> LPTSNPAQELEARQLGRTTRDDLINGNSASCADVIFIYARGSTETGNLGTLGPSIASNLESAFGKDGVWIQGVGGAYRATLGDNALPRGTSSAAIREMLGLFQQANTKCPDATLIAGGYSQGAALAAASIE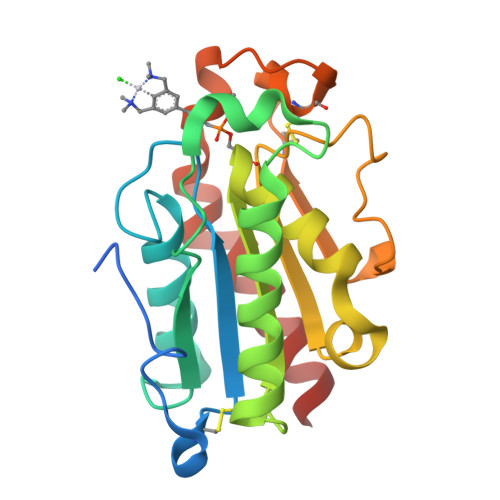DLDSAIRDKIAGTVLFGYTKNLQNRGRIPNYPADRTKVFCKTGDLVCTGSLIVAAPHLAYGPDARGPAPEFLIEKVRAVRGSA Here we describe the determination of the crystal structure of CinA from T. thermophilus (TtCinA), which contains both the NMN deamidase and COG1058 domains and is therefore a bifunctional enzyme. In addition, we show that TtCinA adopts a three-domain structure, with a third, previously unidentified, KH-type domain between the NMN deamidase and COG1058 domains. We demonstrate that TtCinA adopts an asymmetric dimer and present structures with NCN, ADP-ribose, AMP, and ATP bound, which provide experimental validation for the modes of substrate binding proposed previously. We use these structures to propose models for both enzymatic activities and suggest that large scale movement of the COG1058 domains is linked to ADPR catalysis as well as providing a rationale for the usual asymmetric arrangement of the TtCinA dimer.

Data were collected from three different complexes, following soaking of TtCinA crystals with ADP-ribose, ATP, and AMP/ribose 5-phosphate. Both the ADP-ribose and ATP data sets produced clear difference density in both catalytic sites (top and central panels). There was no indication of hydrolysis of ADP-ribose or ATP; this may be due to a slowing of catalysis in the crystalline state. ATP binds in a very similar conformation to ADP-ribose, with the γ-phosphate occupying a location similar to that of the terminal ribose ring. Mg2+ binds between the α- and β-phosphates, as in the ADP-ribose complex. ATP therefore appears to bind in a manner similar to ADP-ribose.

> MERAEILGVGTELLYGETLDTNTAEIARSLKPYALKVERTLRVADEVAPLAREVEEAFARARLVVLSGGLGPTPDDVTREAVALALGEPLELDEAVLGEIEAFFRARGRAMPEANRKQAMRIPSATWLKNPRGTAPGWWVRKGGKDLVLLPGPPPEWRPMWQEVLPRLGLPRRPYAERVLKTWGIGESEIVERLGPLFVREEEEEVGTYPKVHGVEVVVRGREDRVAELAERIKKKLLKEVWGEGEMTLAEAVKRRMEREGATLSTMESLTGGLLGAEITRVPGASRFYLGGVVSYSVGAKARFGVPQDLLSRTVSAETARAMAEAARSLFGSTYALATTGVAGPDPLEGEPPGTVYVALAGPTGAEVRRYRFPGDRETVRLRSVYAALALLVT;> MERAEILGVGTELLYGETLDTNTAEIARSLKPYALKVERTLRVADEVAPLAREVEEAFARARLVVLSGGLGPTPDDVTREAVALALGEPLELDEAVLGEIEAFFRARGRAMPEANRKQAMRIPSATWLKNPRGTAPGWWVRKGGKDLVLLPGPPPEWRPMWQEVLPRLGLPRRPYAERVLKTWGIGESEIVERLGPLFVREEEVEVGTYPKVHGVEVVVRGREDRVAELAERIKKKLLKEVWGEGEMTLAEAVKRRMEREGATLSTMESLTGGLLGAEITRVPGASRFYLGGVVSYSVGAKARFGVPQDLLSRTVSAETARAMAEAARSLFGSTYALATTGVAGPDPLEGEPPGTVYVALAGPTGAEVRRYRFPGDRETVRLRSVYAALALLVT>MSLDVTAKYELIGLMAYPIRHSLSPEMQNKALEKAGLPFTYMAFEVDNDSFPGAIEGLKALKMRGTGVSMPNKQLACEYVDELTPAAKLVGAINTIVNDDGYLRGYNTDGTGHIRAIKESGFDIKGKTMVLLGAGGASTAIGAQGAIEGLKEIKLFNRRDEFFDKALAFAQRVNENTDCVVTVTDLADQQAFAEALASADILTNGTKVGMKPLENESLVNDISLLHPGLLVTECVYNPHMTKLLQQAQQAGCKTIDGYGMLLWQGAEQF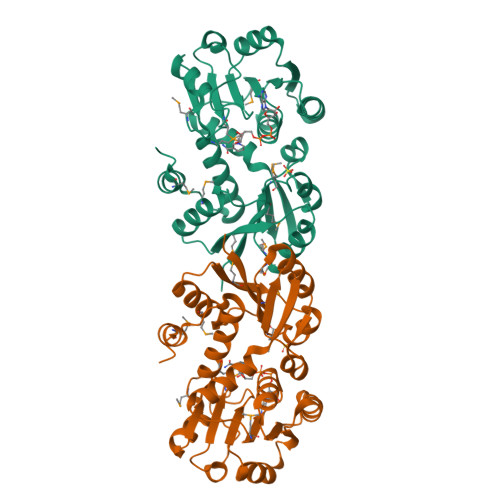TLWTGKDFPLEYVKQVMGFGAEGGSHHHHHH[2x]> MIAAQLLAYYFTELKDDQVKKIDKYLYAMRLSDETLIDIMTRFRKEMKNGLSRDFNPTATVKMLPTFVRSIPDGSEKGDFIALDLGGSSFRILRVQVNHEKNQNVHMESEVYDTPENIVHGSGSQLFDHVAECLGDFMEKRKIKDKKLPVGFTFSFPCQQSKIDEAILITWTKRFKASGVE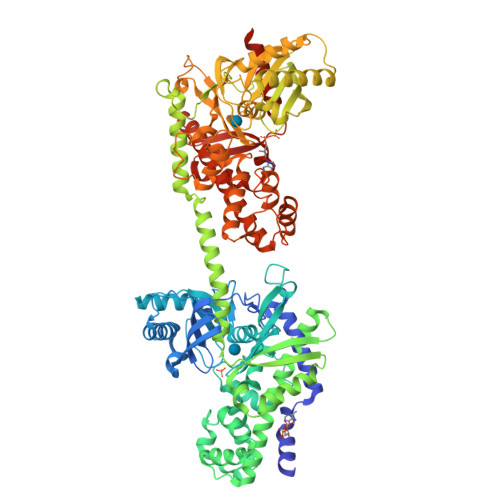GADVVKLLNKAIKKRGDYDANIVAVVNDTVGTMMTCGYDDQHCEVGLIIGTGTNACYMEELRHIDLVEGDEGRMCINTEWGAFGDDGSLEDIRTEFDRAIDAYSLNPGKQLFEKMVSGMYLGELVRLILVKMAKEGLLFEGRITPELLTRGKFNTSDVSAIEKNKEGLHNAKEILTRLGVEPSDDDCVSVQHVCTIVSFRSANLVAATLGAILNRLRDNKGTPRLRTTVGVDGSLYKTHPQYSRRFHKTLRRLVPDSDVRFLLSESGSGKGAAMVTAVAYRLAEQHRQIEETLAHFHLTKDMLLEVKKRMRAEMELGLRKQTHNNAVVKMLPSFVRRTPDGTENGDFLALDLGGANFRVLLVKIRSGKKRTVEMHNKIYAIPIEIMQGTGEELFDHIVSCISDFLDYMGIKGPRMPLGFTFSFPCQQTSLDAGILITWTKGFKATDCVGHDVVTLLRDAIKRREEFDLDVVAVVNDTVGTMMTCAYEEPTCEVGLIVGTGSNACYMEEMKNVEMVEGDQGQMCINMEWGAFGDNGCLDDIRTHYDRLVDEYSLNAGKQRYEKMISGMYLGEIVRNILIDFTKKGFLFRGQISETLKTRGIFETKFLSQIESDRLALLQVRAILQQLGLNSTCDDSILVKTVCGVVSRRAAQLCGAGMAAVVDKIRENRGLDRLNVTVGVDGTLYKLHPHFSRIMHQTVKELSPKCNVSFLLSEDGSGKGAALITAVGVRLRTEASS> THADSLNNLANIKREQGNIEEAVRLYRKALEVFPEFAAAHSNLASVLQQQGKLQEALMHYKEAIRISPTFADAYSNMGNTLKEMQDVQGALQCYTRAIQINPAFADAHSNLASIHKDSGNIPEAIASYRTALKLKPDFPDAYCNLAHCLQIVCDWTDYDERMKKLVSIVADQLEKNRLPSVHPHHSMLYPLSHGFRKAIAERHGNLCLDKINVLHKPPYEHPKDLKLSDGRLRVGYVSSDFGNHPTSHLMQSIPGMHNPDKFEVFCYALSPDDGTNFRVKVMAEANHFIDLSQIPCNGKAADRIHQDGIHILVNMNGYTKGARNELFALRPAPIQAMWLGYPGTSGALFMDYIITDQETSPAEVAEQYSEKLAYMPHTFFIGDHANMFPHLKKKAVIDFKSNGHIYDNRIVLNGIDLKAFLDSLPDVKIVKMKCPDGGDNADSSNTALNMPVIPMNTIAEAVIEMINRGQIQITINGFSISNGLATTQINNKAATGEEVPRTIIVTTRSQYGLPEDAIVYCNFNQLYKIDPSTLQMWANILKRVPNSVLWLLRFPAVGEPNIQQYAQNMGLPQNRIIFSPVAPKEEHVRRGQLADVCLDTPLCNGHTTGMDVLWAGTPMVTMPGETLASRVAASQLTCLGCLELIAKNRQEYED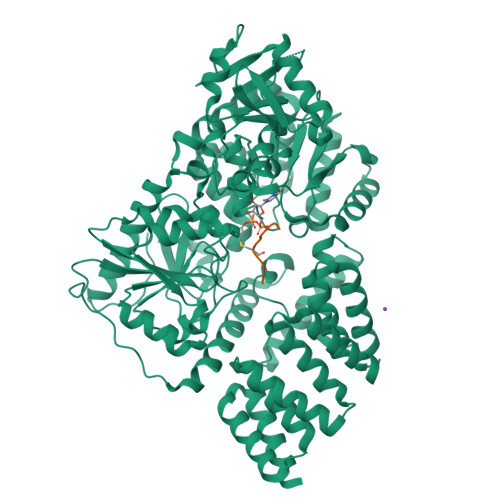IAVKLGTDLEYLKKVRGKVWKQRISSPLFNTKQYTMELERLYLQMWEHYAAGNKPDHMIKPVE>[6x]DELYRQSLEIISRYLREQATGAKDTKPMGRSGATSRKALETLRRVGDGVQRNHETAFQGMLRKLDIKNEDDVKSLSRVMIHVFSDGVTNWGRIVTLISFGAFVAKHLKTINQESCIEPLAESITDVLVRTKRDWLVKQRGWDGFVEFFHVEDLEGGIRNVLLAFAGVAGVGAGLAYLIR;>[6x]DPKKVLDKAKDQAENRVRELKQVLEELYKEARKLDLTQEMRKKLIERYAAAIIRAIGDINNAIYQAKQEAEKLKKAGLVNSQQLDELLRRLDELQKEASRKANEYGREFELKLEYG

Pro-survival homologs (six in humans: Bcl-2, Bcl-xL, Bcl-w, Mcl-1, Bfl-1 and Bcl-B) are structurally similar, but oppose apoptosis by binding and inhibiting Bak and Bax, as well as sequestering pro-apoptotic BH3-only proteins (BOPs). Interactions between BCL2 members are mediated by an amphipathic, helical BH3 motif that recognizes a conserved hydrophobic cleft present in the effectors and pro-survival proteins. Here we describe the computational design and experimental characterization of specific, high affinity protein inhibitors for all six pro-survival BCL2 homologs. As confirmed by biochemical analyses and X-ray crystal structures, the designed proteins engage the BH3-binding grooves of their specific target pro-survival BCL2 family members.

One design, M-CDP04 (subsequently called αMCL1, or anti-Mcl-1), was highly specific for Mcl-1 and bound with picomolar affinity. The crystal structure of the αMCL1•Mcl-1 complex at 2.75 Å resolution reveals how high affinity and specificity were achieved. When Mcl-1 in the design model is superimposed on Mcl-1 in the crystal structure, αMCL1 crystal and design models closely align, highlighting the accuracy of our design calculations (2.1 Å average RMSD among the six separate complexes observed in the asymmetric unit; the N-terminal end of αMCL1 in the crystal structure lying slightly closer to Mcl-1 than in the design). Though the design model does not place αMCL1 near enough to Mcl-1 to make these interactions, the design calculations selected residues with long-range electrostatic complementarity. The BH3-mimetic helix 2 of αMCL1 has three additional helix turns beyond h0 and h4 that have side chains close enough to interact with Mcl-1. These extra contacts, combined with those made by the peripheral helices, expand the classic BH3 interface by 534 Å2. (C) αMCL1 computationally designed residues E111, R108 and N104 complement nearby Mcl-1 residues. (D) αMCL1 residue 46 was redesigned from glutamate (BINDI scaffold) to isoleucine to accommodate the hydrophobic Mcl-1 binding pocket. (E) Designed residues R42, K43 and K44 promote long-range electrostatic complementarity to the negatively-charged loop region of Mcl-1. αMCL1 residue E47 (borrowed from Bim) makes ionic interactions with Mcl-1 residues S245 and R248. (F) Designed residues K68, Q69, and E72, and Bim residue N62, make polar interactions with the Mcl-1 backbone.> GHMLRHIQNSLGSVYRSNTATPQGQII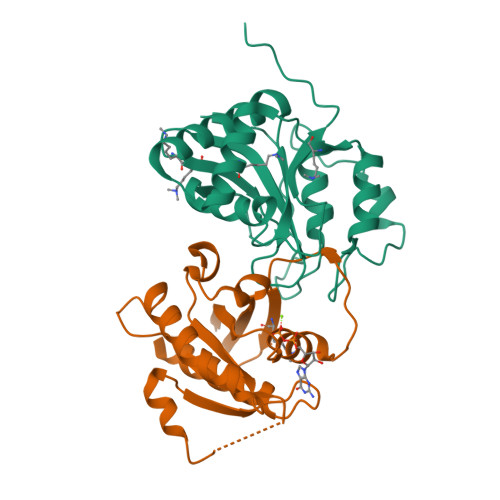HHRNFQSQFDTTGNTLYNNAWVCSLNVIKSRDGNNYSALEDITSDNQAFNNILEGIDIIECENLLKEMNVQKIPESSLFTNIKEALQAEVFNSTVEDDFESFISYELQNHGPLMLIRPSLGSECLHAECIVGYDSEVKKVLIYDSMNTSPEWQSNIDVYDKLTLAFNDKYKNEDCSICGLYYDGVYEPKPLHSSSWKDWCTIL;> METREHLFKVLVIGELGVGKTSIIKRYVHQLFSQHYRATIGVDFALKVLNWDSRTLVRLQLWDIAGQERFGNMTRVYYKEAVGAFVVFDISRSSTFEAVLKWKSDLDSKVHLPNGSPIPAVLLANKCDQNKDSSQSPSQVDQFCKEHGFAGWFETSAKDNINIEEAARFLVEKILVNHQSFPN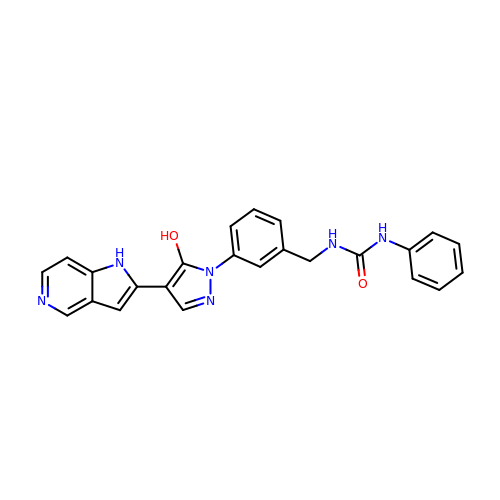1-[[3-[5-hydroxy-4-(1H-pyrrolo[3,2-c]pyridin-2-yl)pyrazol-1-yl]phenyl]methyl]-3-phenylurea | C24 H20 N6 O2 | YWSHOZUTPIGEGZ-UHFFFAOYSA-N To investigate protein HHP adaptation, Elastic Incoherent Neutron Scattering (EINS) and Quasi-Elastic Neutron Scattering (QENS) have been employed to study the dynamics of two orthologous proteins from T. barophilus (Tba) and T. kodakarensis (Tko), which only differ by their optimal growth pressure. X-ray crystallography was performed to obtain the structures of the proteins. Both present very similar features: their structure is dominated by β-sheet contributions with turns and disordered regions connecting them, forming a jelly-roll barrel structure, and both present a dimeric quaternary structure. The active site is located in a pocket inside the barrel and is conserved between the two proteins (His44, His46, Glu51 and His85). The two orthologs differ at 16 positions, and most of the substitutions are located at the protein–water interface and involve mainly polar and charged residues, with the notable exceptions of I35V, located in the hydrophobic core of the protein, and I100V, located at the monomer–monomer interface.

Interestingly, the catalytic metal ion coordinated by these four residues is found to be magnesium in Tba PMI and zinc in Tko PMI; however, the structure’s resolution does not allow for making a definitive assignment, as the Van der Waals radius of both ions is smaller than the resolution. Tko PMI crystals were obtained after one week from condition E8 of the Structure screen 1 + 2 kit (Molecular Dimensions), containing 0.2 M ammonium phosphate monobasic, 0.1 M Tris pH 8.5, and 50% v/v MPD. Tba PMI crystals belong to the I222 space group and contain one molecule in the asymmetric unit, while Tko PMI crystals belong to the P31 space group and contain eight molecules in the asymmetric unit. After model building using Coot and Refine from the Phenix package (Tba PMI) or REFMAC5 (Tko PMI), the final structures exhibited an R(%)/R(%)free of 0.18/0.20 at 1.7 Å (Tba PMI) and 0.23/0.29 at 2.2 Å (Tko PMI). Hence, our data indicate that the extent of compression of the protein hydrophobic core is larger in Tko PMI than in Tba PMI, presumably due to the presence of bigger cavities in the former. The appearance of VFT behaviour on such a fast time-scale is intriguing, and it shows that side-chain relaxations are strongly coupled to hydration water dynamics in Tko PMI. It appears that Tko PMI’s dynamics are dominated by cooperative motions and that high pressure can destabilize them, as highlighted by the increase in fragility (i.e., decreasing D) with increasing pressure, while Tba PMI’s dynamics are dominated by pressure-insensitive activated processes. On the other hand, the temperature dependence of Tko PMI appears to be stronger, and a sizeable increase in the confinement radius is detected with increasing pressure.

>MKAEIKNLIDRGTYRKLPLFEGELPEGSYAQIVEVKPKQTVKKHYHERQYELFYIISGEARLGIGDTEYQAKPGDIFLVKPKTVHWVVNEKDEPFRLFVVKLNYHGDDSVWLEGSF[4x];> AEIKNLIDRGTYRKLPLFEGELPEGSYAQIVEVKPKQTVKKHYHERQYELFYIISGEARLGIGDTEYQAKPGDIFLVKPKTVHWVVNEKDEPFRLFVVKLNYHGDDSVWLEGSF;>[2x]NLIDRGTYRKLPLFEGELPEGSYAQIVEVKPKQTVKKHYHERQYELFYIISGEARLGIGDTEYQAKPGDIFLVKPKTVHWVVNEKDEPFRLFVVKLNYHGDDSVWLEGSF;> GTYRKLPLFEGELPEGSYAQIVEVKPKQTVKKHYHERQYELFYIISGEARLGIGDTEYQAKPGDIFLVKPKTVHWVVNEKDEPFRLFVVKLNYHGDDSVWLEGSF> MARDPLPFFPPLYLGGPEITTENCEREPIHIPGSIQPHGALLTADGHSGEVLQVSLNAATFLGQEPTVLRGQTLAALLPEQWPALQAALPPGCPDALQYRATLDWPAAGHLSLTVHRVAELLILEFEPTEAWDSIGPHALRNAMFALESAPNLRALAEVATQTVRELTGFDRVMLYKFAPDATGEMIAEARREGMQAFLGHRFPASHTPAQARALYTRHLLRLTADTRAAAVP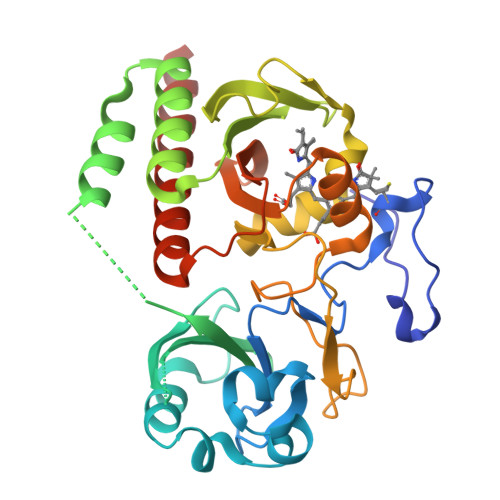LDPVLNPQTNAPTPLGGAVLRATSPMHMQYLRNMGVGSSLSVSVVVGGQLWGLIVCHHQTPYVLPPDLRTTLEELGRKLSGQVQRKEALEHHHHHH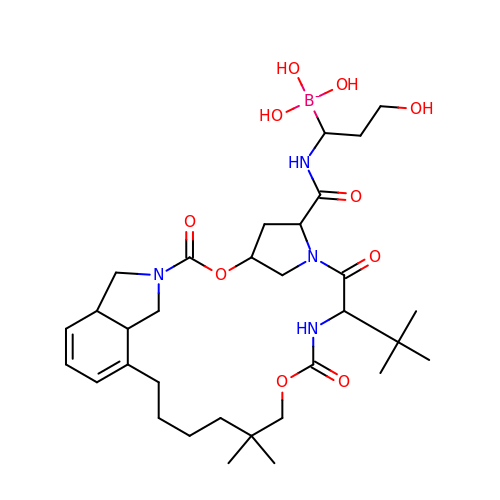(1-{[(10-tert-butyl-15,15-dimethyl-3,9,12-trioxo-6,7,9,10,11,12,14,15,16,17,18,19,23,23a-tetradecahydro-1H,5H-2,23:5,8-dimethano-4,13,2,8,11-benzodioxatriazacyclohenicosin-7(3H)-yl)carbonyl]amino}-3-hydroxypropyl)(trihydroxy)borate(1-) | C32 H52 B N4 O10 | TWUMYENOHGWFCN-UHFFFAOYSA-N> ALCKFCDVRFSTCDNQKSCMSNCSITSICEKPQEVCVAVWRKNDENITLETVCH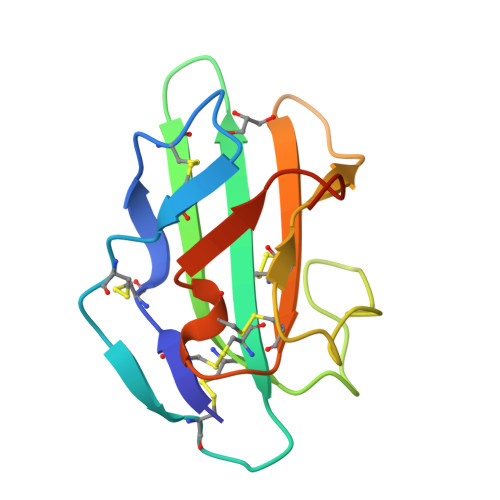DPKLPYHDFILEDAASPTCIMKEKKKPGETFFMCSCSSDECNDNIIFSEEYNTSNPD>[16x]GAMANPPVFTTSQGCPVSDPFTTQRIPLDSTGYKYAPPIGPLLLQDFKLIDTLSHFDRERIPERVVHAKGAGAYGVFEVTDDITDVCSAKFLDTVGKKTRIFTRFSTVGGEKGSADTARDPRGFATKFYTEDGNLDLVYNNTPIFFIRDPIKFPHFIHTQKRNPATNLKDPNMFWDYLTANDESLHQVMYLFSNRGTPASYRTMNGYSGHTYKWYNSKGEW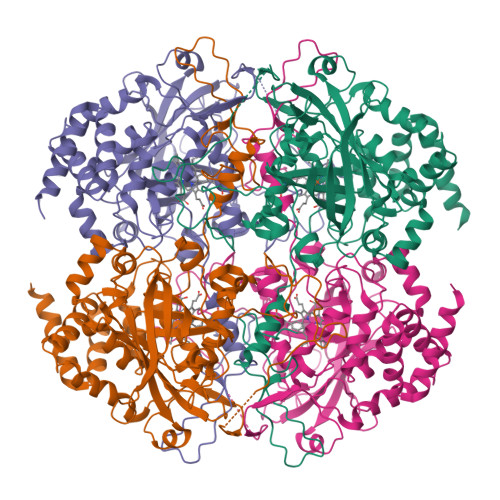VYVQVHFIANQGVHNLLDEEAGRLAGEDPDHSTRDLWEAIEKGDYPSWECYIQTMTLEQSKKLPFSVFDLTKVWPHKDFPLRHFGRFTLNENPKNYYAETEQIAFSPSHTVPGMEPSNDPVLQSRLFSYPDTHRHRLGPNYHQIPVNCPLKSGSFNPINRDGPMCVDGNLGGTPNYANAYNCPIQYAVSPKASGNKPDEKYTGEVVPYHWEHTDYDYFQPKMFWKVLGRTPGEQESLVKNVANHVSAADEFIQDRVYEYFSKAEPIIGDLIRKKVQELKRKASSPSKI>[2x]SNIGSGGSQIDGFVRTLRARPEAGGKVPVFVFHPAGGSTVVYEPLLGRLPADTPMYGFERVEGSIEERAQQYVPKLIEMQGDGPYVLVGWSLGGVLAYACAIGLRRLGKDVRFVGLIDAVRAGEEIPQTKEEIRKRWDRYAAFAEKTFNVTIPAIPYEQLEELDDEGQVRF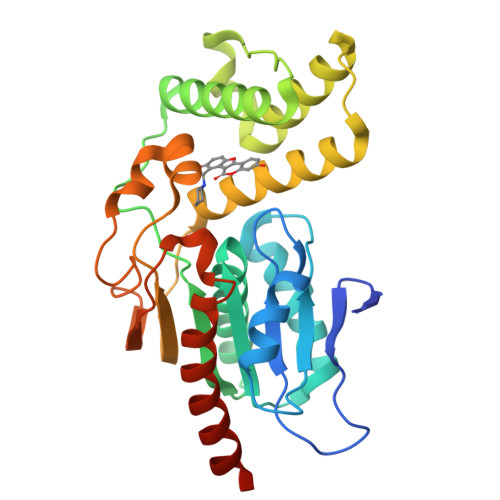VLDAVSQSGVQIPAGIIEHQRTSYLDNRAIDTAQIQPYDGHVTLYMADRYHDDAIMFEPRYAVRQPDGGWGEYVSDLEVVPIGGEHIQAIDEPIIAKVGEHMSRALGQIEADRTSEVGKQ> MEEFQQIPDFYGCYLLQSISKRQSFYIGSTPNPVRRLRQHNGSLSRGGAYRTKRDGTRPWEMVAIVYGFPSRIAALQFQHAWQHGYQTRYIKSQDRVVKTRKGGRSIHHKLAMITSLLKNEYFRYMDLTLHFFNQKVEEIWKNDKFNVSQTQESIDNNYTVSLSQDALTEINNDTIDDIMDVNEKNMELVQNLYSTTLAEKTKTLLLYKEKIDTGINTCQFCNKIIKHNLSGNISENLFAFCRDTSCTFVSHLACAYRYFMSNTELPKEDTIIPQSPKCPKCYTLLKWCDVIYYSIKLNKDNTTADDKKKTI;> SNQKKVGVTSKSEVFEFLTHLVKQEPDL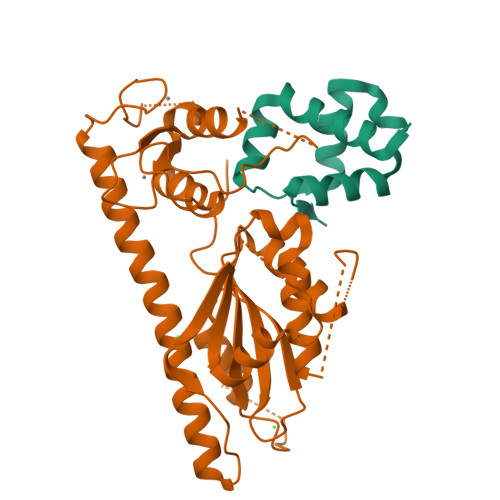LTRIYCFQPITMNDLINKLRNKDSFVDLIDDGTIREWTDKLGICIRSNNLKD> QAQITGRPEWIWLALGTALMGLGTLYFLVKGMGVSDPDAKKFYAITTLVPAIAFTMYLSMLLGYGLTMVPFGGEQNPIYWARYADWLFTTPLLLLDLALLVDADQGTIL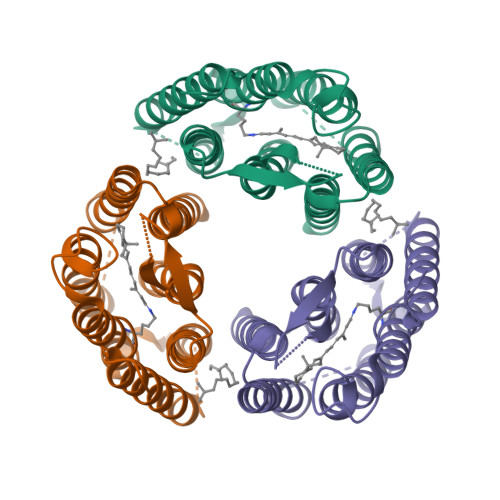ALVGADGIMIGTGLVGALTKVYSYRFVWWAISTAAMLYILYVLFFGFTSKAESMRPEVASTFKVLRNVTVVLWSAYPVVWLIGSEGAGIVPLNIDTLLFMVLDVSAKVGFGLILLRSRAIFGEAEAPEPSAGDGAAATSD> MLLKFTEDAWADYCYWQNQDKKTLKRINKLIKDIQRDPFTGIGKPEPLKYDYQGAWSRR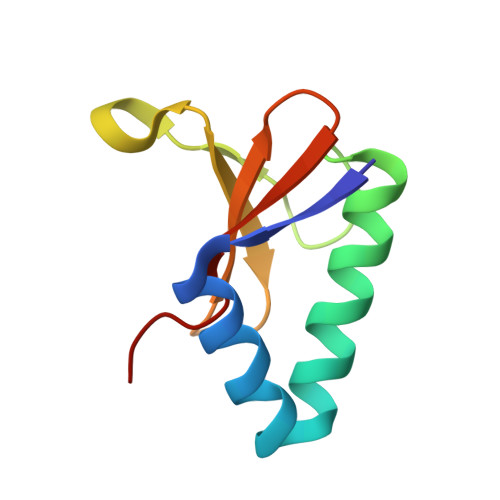IDAENRLIYMMDGDSVAFLSFKDHY> IINGEDCSPHSQPWQAALVMENELFCSGVLVHPQWVLSAAHCFQNSYTIGLGLHSLEADQEPGSQMVEASLSVRHPEYNRPLLANDLMLIKLDESVSESDTIRSISIASQCPTAGNSCLVSGWGLLANGRMPTVLQCVNVSVVSEEVCSKLYDPLYHPSMFCAGGGQDQKDSCNGDSGGPLICNGYLQGLVSFGKAPCGQVGVPGVYTNLCKFTEWIEKTVQA;> GSSVVVDTNGQPVSNGADAYYLVPVSHGHAGLALAKIGNEAEPRAVVLDPHHRPGLPVRFESPLDINIIKESYFLN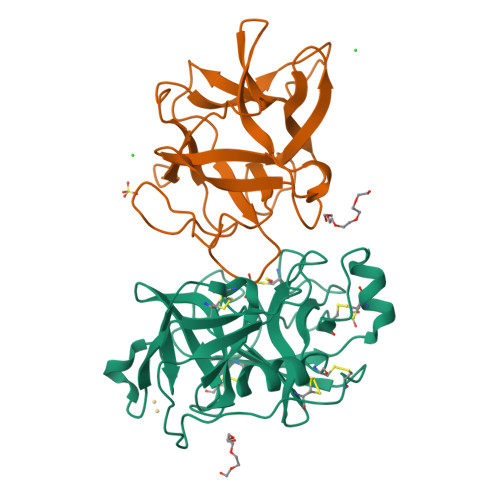IKFGPSSSDSGVWDVIQQDPIGLAVKVTDTKSLLGPFKVEKEGEGYKIVYYPERGQTGLDIGLVHRNDKYYLAVKDGEPCVFKIRKATDE>[3x]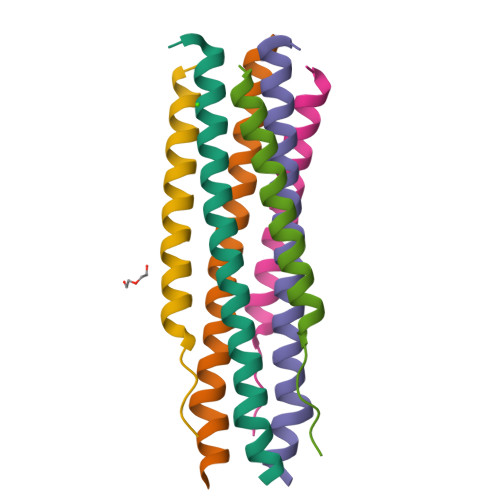XQARSDIEKLKEAIRDTNKAVQSVQSSIGNLIVAIKSVQDYVNKEIVPSIARX;>[3x]XVALDPIDISIVLNKIKSQLEESKEWIRRSNKILDSIX> MEGESSISIGYAQSRVKEDGYKLDKNPRGFNLKYRYEFNNDWGVIGSFAQTRRGFEE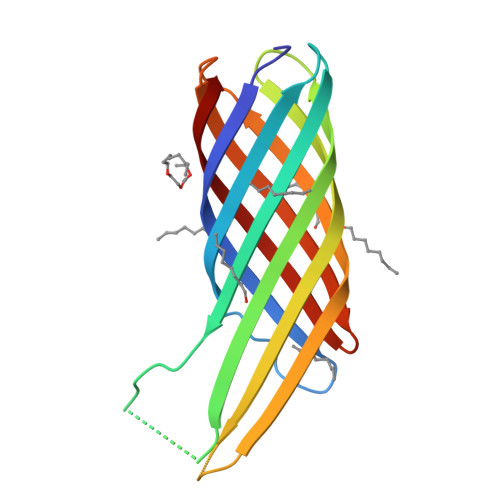SVDGFKLIDGDFKYYSVTAGPVFRINEYVSLYGLLGAGHGKAKFSSIFGQSESRSKTSLAYGAGLQFNPHPNFVIDASYEYSKLDDVKVGTWMLGAGYRF>[8x]MRRSHTIGVVTTGLSFYGPSQILVGIERAAREHGYSLLLATVHEDPDEVEEAINTLRERRVDGIIIVAPHNSEEEAQLAQEAGVPPVVFLSAQPPGVPTVSVDQYAGARLATEH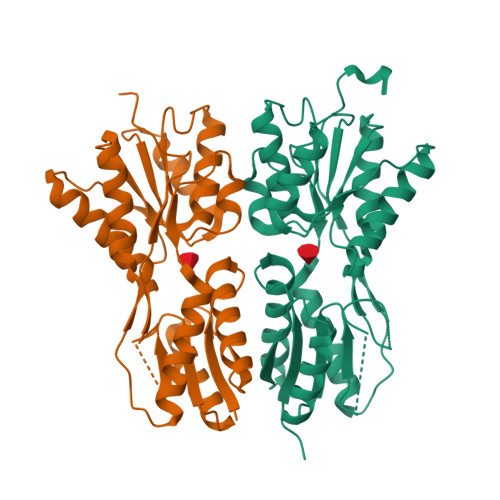LLDLGHRRIALITGPQDWLEARERLQGWREALAEAGLPPPAVLQGDWSAASGYEAARQLLEQPDFTAIFAANDQMALGVLRALHERGLRVPDDVSVVGFDDIPESAYFHPPLTTVRQDFEELGRQAVEQLLEMIEGEEPPPPAVLPPELIVRESTAPPENLYFQGL>[2x]MKHTLPDLPFDYADLEPVISHEIMQLHHQKHHATYVNNLNQIEEKLHEAVSKGNLKEAIALQPALKFNGGGHINHSIFWTNLA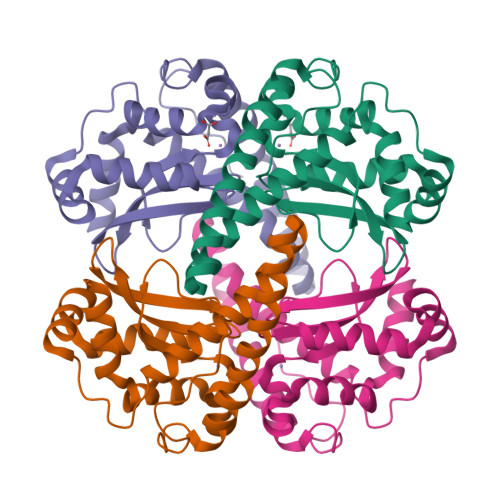KDGGEPSKELMDTIKRDFGSLDNLQKRLSDITIAVQGSGWGWLGYCKKDKILKIATCANQDPLEGMVPLFGIDVWEHAYYLQYKNVRPDYVHAIWKIANWKNISERFANARQ> GPGDPHTYEDPNQAVLKFTTEIHPSCVTRQKVIGAGEFGEVYKGMLKTSSGKKEVPVAIKTLKAGYTEKQRVDFLGEAGIMGQFSHHNIIRLEGVISKYKPMMIITEYMENGALDKFLREKDGEFSVLQLVGMLRGIAAGMKYLANMNYVHRDLAARNILVNSNLVCKVSDFGLSRVLEDDPEATYTTSGGKIPIRWTAPEAISYRKFTSASDVWSFGIVMWEVMTYGER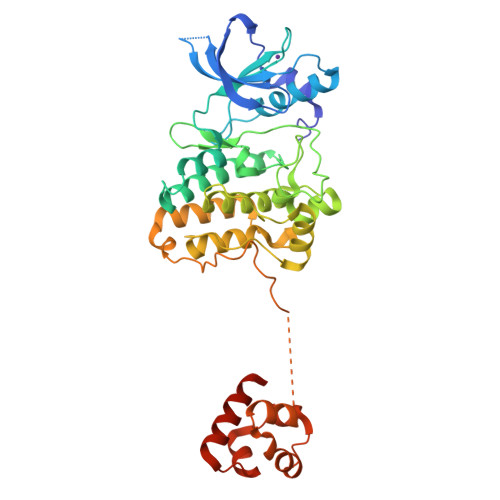PYWELSNHEVMKAINDGFRLPTPMDCPSAIYQLMMQCWQQERARRPKFADIVSILDKLIRAPDSLKTLADFDPRVSIRLPETSGEEGVPFRTVSEWLESIKMQQYTEHFMAAGYTAIEKVVQMTNDDIKRIGVRLPGHQKRIAYSLLGLKDQVNTVGIPI> SPSVEACGYSDRVAQLTVGNSTITTQEAANIVLSYGEWPEYCPSTDATAVDKPTRPDVSVNRFYTLSTKSWKTESTGWYWKFPDVLNDTGVFGQNAQFHYLYRSGFCMHVQCNASKFHQGALLVAAIPEFVIAASSPATKPNGRGLYPDFAHTNPGKDGQEFRDPYVLDAGIPLSQALVFPHQWINLRTNNCATIIMPYVNALPFDSALNHSNFGLVVIPISPLKYCN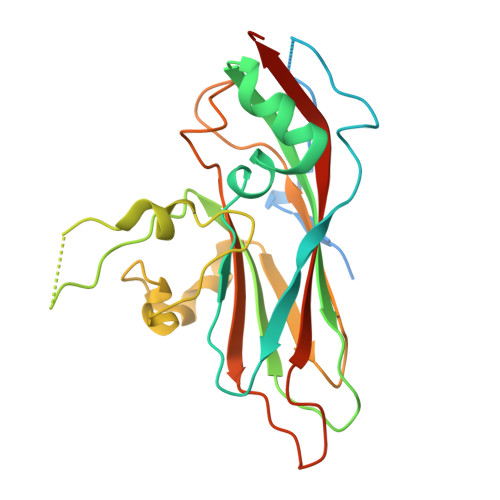GATTEVPVTLTIAPLNSEFSGLRQAIKQ> MAHHHHHHMSQLSTIIEQAFEDRANFTAADCPSEIRQAVEEAIAGLDNGTLRVAEKINGEWVVHQWLKKAVLLSFKLNDNKPIESCDLRFYDKVETKFSGWTEEQFKAAGVRVVPPAVARRGSFQAKNVVLMPSYVNIGAYVDEGTMVDTWATVGSCAQIGKNVHLSGGVGIGGVLEPLQANPTIIEDNCFIGARSEIVEGVIVEEGSVISMGVYIG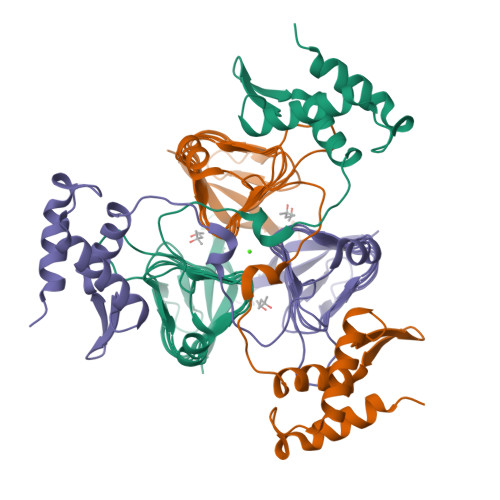QSTRIYDRETGEIHYGRVPAGSVVVPGNLPSADGKYSLYAAIIVKKVDAQTRAKTSLNDLLRAD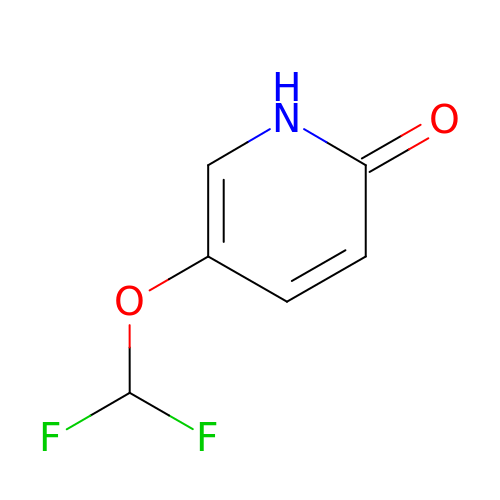5-(difluoromethoxy)pyridin-2(1H)-one | C6 H5 F2 N O2 | VRWFXRMPZMWPKH-UHFFFAOYSA-N> SSPGQLTLLQ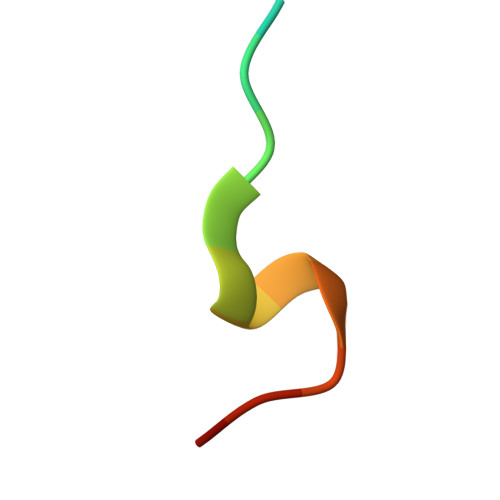CGFSK>MPPGKCLFSGVFCNMAEKQTAKRNRREEILQSLALMLESSDGSQRITTAKLAASVGVSEAALYRHFPSKTRMFDSLIEFIEDSLITRINLILKDEKDTTARLRLIVLLILGFGERNPGLTRILTGHALMFEQDRLQGRINQLFERIEVQLRQVMREKKMREGEGYTLDETLLASQLLA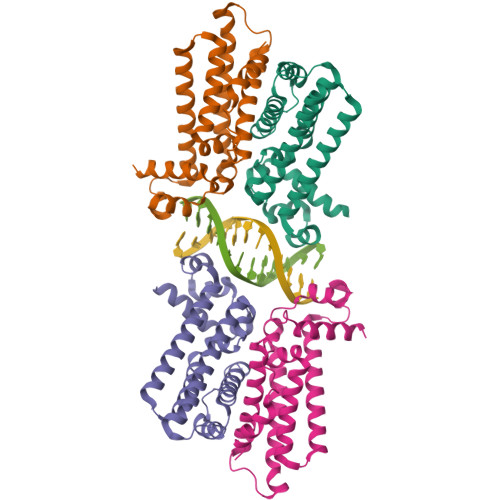FCEGMLSRFVRSEFKYRPTDDFEARWPLVAAQLQ[4x]(2R)-2-[(1S)-1-(benzoylamino)-1-methoxy-2-oxoethyl]-5-methylidene-5,6-dihydro-2H-1,3-thiazine-4-carboxylic acid | C16 H16 N2 O5 S | 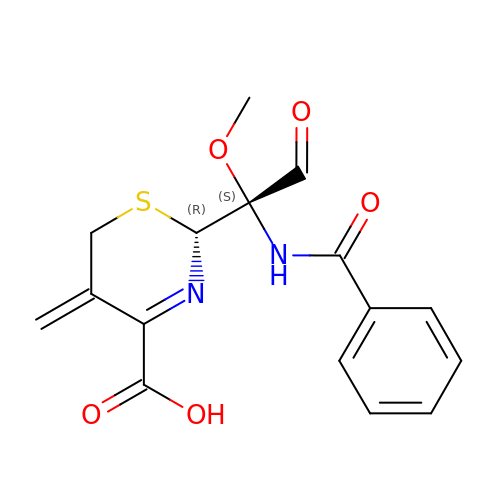DDPBNTJUSOYARI-CVEARBPZSA-N>AGAIENARKEIKRISLEDHAESEYGAIYSVSGPVVIAENMIGCAMYELVKVGHDNLVGEVIRIDGDKATIQVYEETAGLTVGDPVLRTGKPLSVELGPGLMETIYDGIQRPLKAIKEESQSIYIPRGIDTPALDRTIKWQFTPGKFQVGDHISGGDIYGSVFENSLISSHKILLPPRSRGTITWIAPAGEYTLDEKILEVEFDGKKSDFTLYHTWPVRVPRPVTEKLSADYPLLTGQRVLDALFPCVQGGTTCIPGAFGCGKTVISQSLSKYSNSDAIIYVGCGERGNEMAEVLMEFPELYTEMSGTKEPIMKRTTLVANTSNMPVAAREASIYTGITLAEYFRDQGKNVSMIADSSSRWAEALREISGRLGEMPADQGFPAYLGAKLASFYERAGKAVALGSPDRTGSVSIVAAVSPAGGDFSDPVTTATLGITQVFWGLDKKLAQRKHFPSINTSVSYSKYTNVLNKFYDSNYPEFPVLRDRMKEILSNAEELEQVVQLVGKSALSDSDKITLDVATLIKEDFLQQNGYSTYDAFCPIWKTFDMMRAFISYHDEAQKAVANGANWSKLADSTGDVKHAVSSSKFFEPSRGEKEVHGEFEKLLSTMQERFAESTD[3x];>[3x]MVLSDKELFAINKKAVEQGFNVKPRLNYNTVSGVNGPLVILEKVKFPRYNEIVNLTLPDGTVRQGQVLEIRGDRAIVQVFEGTSGIDVKKTTVEFTGESLRIPVSEDMLGRIFDGSGRPIDNGPKVFAEDYLDINGSPINPYARIYPEEMISTGVSAIDTMNSIARGQKIPIFSASGLPHNEIAAQICRQAGLVRPTKDVHDGHEENFSIVFAAMGVNLETARFFKQDFEENGSLERTSLFLNLANDPTIERIITPRLALTTAEYLAYQTERHVLTILTDMSSYADALREVSAAREEVPGRRGYPGYMYTDLSTIYERAGRVEGRNGSITQIPILTMPNDDITHPIPDLTGYITEGQIFVDRQLHNKGIYPPINVLPSLSRLMKSAIGEGMTRKDHGDVSNQLYAKYAIGKDAAAMKAVVGEEALSIEDKLSLEFLEKFEKTFITQGAYEDRTVFESLDQAWSLLRIYPKEMLNRISPKILDEFYDRARDDADEDEEDPDTRSSGKKKDASQEESLI;>MSSAITALTPNQVNDELNKMQAFIRKEAEEKAKEIQLKADQEYEIEKTNIVRNETNNIDGNFKSKLKKAMLSQQITKSTIANKMRLKVLSAREQSLDGIFEETKEKLSGIANNRDEYKPILQSLIVEALLKLLEPKAIVKALERDVDLIESMKDDIMREYGEKAQRAPLEEIVISNDYLNKDLVSGGVVVSNASDKIEINNTLEERLKLLSEEALPAIRLELYGPSKTRKFFD[3x];>[3x]MSQKNGIATLLQAEKEAHEIVSKARKYRQDKLKQAKTDAAKEIDSYKIQKDKELKEFEQKNAGGVGELEKKAEAGVQGELAEIKKIAEKKKDDVVKILIETVIKPSAEVHINAL;> MSGNREQ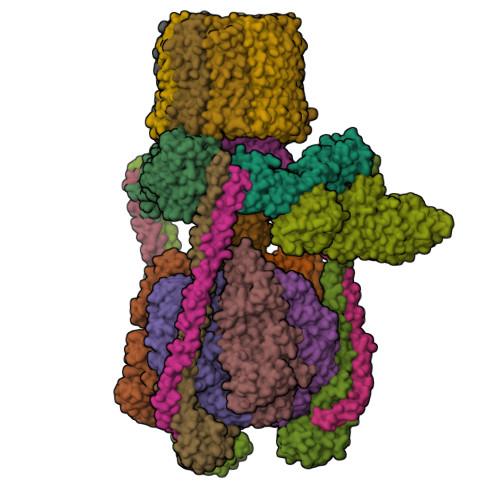VFPTRMTLGLMKTKLKGANQGYSLLKRKSEALTKRFRDITKRIDDAKQKMGRVMQTAAFSLAEVSYATGENIGYQVQESVSTARFKVRARQENVSGVYLSQFESYIDPEINDFRLTGLGRGGQQVQRAKEIYSRAVETLVELASLQTAFIILDEVIKVTNRRVNAIEHVIIPRTENTIAYINSELDELDREEFYRLKKVQEKKQNETAKLDAEMKLKRDRAEQDASEVAADEEPQGETLVADQEDDVIF;> MAEKRTLIAVIADEDTTTGLLLAGIGQITPETQEKNFFVYQEGKTTKEEITDKFNHFTEERDDIAILLINQHIAENIRARVDSFTNAFPAILEIPSKDHPYDPEKDSVLKRVRKLFGE;> MATALYTANDFILISLPQNAQPVTAPGSKTDSWFNETLIGGRAFVSDFKIPEFKIGSLDTLIVESEELSKVDNQIGASIGKIIEILQGLNETSTNAYRTLPINNMPVPEYLENFQWQTRKFKLDKSIKDLITLISNESSQLDADVRATYANYNSAKTNLAAAERKKTGDLSVRSLHDIVKPEDFVLNSEHLTTVLVAVPKSLKSDFEKSYETLSKNVVPASASVIAEDAEYVLFNVHLFKKNVQEFTTAAREKKFIPREFNYSEELIDQLKKEHDSAASLEQSLRVQLVRLAKTAYVDVFINWFHIKALRVYVESVLRYGLPPHFNIKIIAVPPKNLSKCKSELIDAFGFLGGNAFMKDKKGKINKQDTSLHQYASLVDTEYEPFVMYIINL;> MGATKILMDSTHFNEIRSIIRSRSVAWDALARSEELSEIDASTAKALESILVKKNIGDGLSSSNNAHSGFKVNGKTLIPLIHLLSTSDNEDCKKSVQNLIAELLSSDKYGDDTVKFFQEDPKQLEQLFDVSLKGDFQTVLISGFNVVSLLVQNGLHNVKLVEKLLKNNNLINILQNIEQMDTCYVCIRLLQELAVIPEYRDVIWLHEKKFMPTLFKILQRATDSQLATRIVATNSNHLGIQLQYHSLLLIWLLTFNPVFANELVQKYLSDFLDLLKLVKITIKEKVSRLCISIILQCCSTRVKQHKKVIKQLLLLGNALPTVQSLSERKYSDEELRQDISNLKEILENEYQELTSFDEYVAELDSKLLCWSPPHVDNGFWSDNIDEFKKDNYKIFRQLIELLQAKVRNGDVNAKQEKIIIQVALNDITHVVELLPESIDVLDKTGGKADIMELLNHSDSRVKYEALKATQAIIGYTFK;> MEGVYFNIDNGFIEGVVRGYRNGLLSNNQYINLTQCDTLEDLKLQLSSTDYGNFLSSVSSESLTTSLIQEYASSKLYHEFNYIRDQSSGSTRKFMDYITYGYMIDNVALMITGTIHDRDKGEILQRCHPLGWFDTLPTLSVATDLESLYETVLVDTPLAPYFKNCFDTAEELDDMNIEIIRNKLYKAYLEDFYNFVTEEIPEPAKECMQTLLGFEADRRSINIALNSLQSSDIDPDLKSDLLPNIGKLYPLATFHLAQAQDFEGVRAALANVYEYRGFLETGNLEDHFYQLEMELCRDAFTQQFAISTVWAWMKSKEQEVRNITWIAECIAQNQRERINNYISVY;>MTELCPVYAPFFGAIGCASAIIFTSLGAAYGTAKSGVGICATCVLRPDLLFKNIVPVIMAGIIAIYGLVVSVLVCYSLGQKQALYTGFIQLGAGLSVGLSGLAAGFAIGIVGDAGVRGSSQQPRLFVGMILILIFAEVLGLYGLIVALLLNSRATQDVVC[10x];> MAEKEEAIFRSAEMALVQFYIPQEISRDSAYTLGQLGLVQFRDLNSKVRAFQRTFVNEIRRLDNVERQYRYFYSLLKKHDIKLYEGDTDKYLDGSGELYVPPSGSVIDDYVRNASYLEERLIQMEDATDQIEVQKNDLEQYRFILQSGDEFFLKGDNTDSTSYMDEDMIDANGENIAAAIGASVNYVTGVIARDKVATLEQILWRVLRGNLFFKTVEIEQPVYDVKTREYKHKNAFIVFSHGDLIIKRIRKIAESLDANLYDVDSSNEGRSQQLAKVNKNLSDLYTVLKTTSTTLESELYAIAKELDSWFQDVTREKAIFEILNKSNYDTNRKILIAEGWIPRDELATLQARLGEMIARLGIDVPSIIQVLDTNHTPPTFHRTNKFTAGFQSICDCYGIAQYREINAGLPTIVTFPFMFAIMFGDMGHGFLMTLAALSLVLNEKKINKMKRGEIFDMAFTGRYIILLMGVFSMYTGFLYNDIFSKTMTIFKSGWKWPDHWKKGESITATSVGTYPIGLDWAWHGTENALLFSNSYKMKLSILMGFIHMTYSYFFSLANHLYFNSMIDIIGNFIPGLLFMQGIFGYLSVCIVYKWAVDWVKDGKPAPGLLNMLINMFLSPGTIDDELYPHQAKVQVFLLLMALVCIPWLLLVKPLHFKFTHKKKSHEPLPSTEADASSEDLEAQQLISAMDADDAEEEEVGSGSHGEDFGDIMIHQVIHTIEFCLNCVSHTASYLRLWALSLAHAQLSSVLWTMTIQIAFGFRGFVGVFMTVALFAMWFALTCAVLVLMEGTSAMLHSLRLHWVESMSKFFVGEGLPYEPFAFEYKDMEVAVASASSSASS> NSSILSLCAFSVDPKKTYLDFIQQGGTPIANCVKMLCDHAGTGMAITVKPDATTSQDSYGGASVCIYCRARVEHPDVDGLCKLRGKFVQVPVGIKDPVSYVL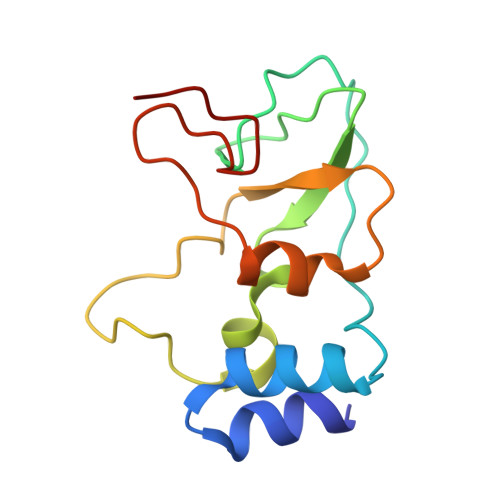THDVCRVCGFWRDGSCSCVS> RAKKPRKARTAFSDHQLNQLERSFERQKYLSVQDRMDLAAALNLTDTQVKTWYQNRRTKWKRQTAV

Transcription factors (TFs) recognize specific bases within their DNA-binding motifs, with each base contributing nearly independently to total binding energy. However, the energetic contributions of particular dinucleotides can deviate strongly from the additive approximation, indicating that some TFs can specifically recognize DNA dinucleotides. Here we solved high-resolution (<1 Å) structures of MYF5 and BARHL2 bound to DNAs containing sets of dinucleotides that have different affinities to the proteins. The dinucleotides were recognized either enthalpically, by an extensive water network that connects the adjacent bases to the TF, or entropically, by a hydrophobic patch that maintained interfacial water mobility.

One BARHL2–DNAAC crystal diffracted to 0.95 Å, which is thus far the highest resolution for any TF–DNA complex. The high resolution revealed alternative conformations for most of the phosphates, sugars and bases of the DNA backbone, hitherto only observed in two previous TF–DNA complexes. We first assessed whether differences in resolution would affect the detection of the water molecules using the two BARHL2–DNAAC structures solved at 0.95 Å and 1.3 Å. Although overall more water molecules are seen in the protein–DNA interface in the 0.95 Å structure, inspection of the water content at the site of the variant dinucleotide at both resolutions showed conserved positions of all of the ten water molecules, indicating that at this range, resolution does not substantially affect detection of water molecules contributing to recognition of the dinucleotide. Analysis of the highest-affinity complex, BARHL2–DNAAC, revealed that the high-affinity binding of BARHL to DNAAC is caused by a combination of indirect and direct recognition of DNA. Key amino acids involved in the recognition of the AC dinucleotide and its complementary bases are Asn282 and two threonines: Thr278 and Thr285. Thr278 is connected to DNA by two water chains. The first water chain contains three water molecules that together connect the side-chain oxygen of Thr278 with the side-chain oxygen of Asn282 and N7 of the A of the AC dinucleotide (A7). On the other side, Thr278 is connected to N4 of the C of AC (C8) by a second chain of four water molecules.> E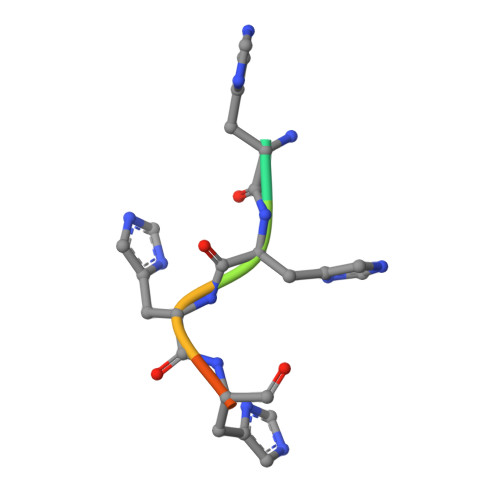HHHHHH>[4x]GHMRNVMLITGASRGIGAATALLAAERGYAVVLNYLRNREAAEALRQRIERQGGEALAVAADVAEE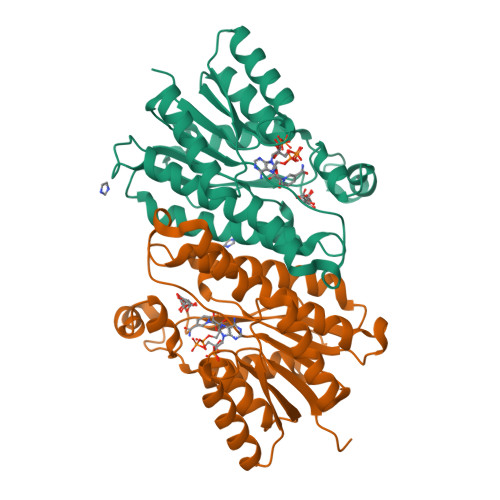GDVERLFASIDERFGRLDVLVNNAGMLEAQTRLENIDAARLHRVFATNVTGSFLCAREAVKRLSTRHGGRGGSIVNVSSMASRLGSPNEYIDYAAAKGAIDSMTIGLAREVAAEGIRVNAVRPGLIDTEIHASGGEPGRIERLKGGIPLGRGGTAEEVARAILWLASDEASYSTGTFIDVSGGR> MADRLTQLQDAVNSLADQFCNAIGVLQQCGPPASFSNIQTAINKDQPANPTEEYAQLFAALIARTAKDIDVLIDSLPSEESTAALQAASLYKLEEENHEAATCLEDVVYRGDMLLEKIQSALADIAQSQLKTRS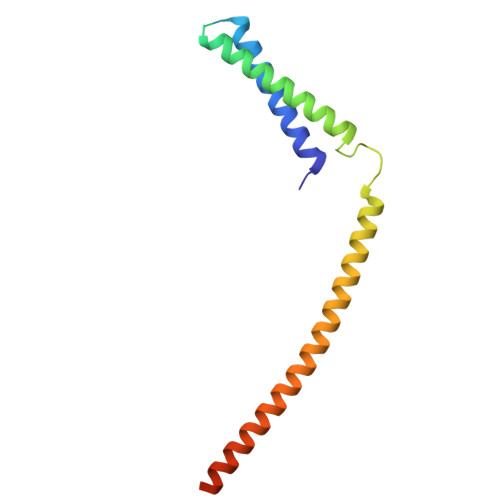VTHSHSLPDS> XXXXXXXXXXXXXXXXXXXXXXXXXXXXXXXXXXXXXXXXXXXXXXXXXXXXXXXXXXXXXXXXXXXXXXXXXXXXXXXXXXXXXXXXXXXXXXXXXXXXXXXXXXXXXXXXXXXXXXXXXXXXXXXXXXXXXXXXXXXXXXXXXXXXXXXXXXXXXXXXXXXXXXXXXXXXXXXXXXXXXXXXXXXXXXPSVPECFTIEKKSSYFIIEPQDLSTKVASICGVIVPKVHTIHDKVFYPLTFVPTHKTVSSLRQLGRKIQNSTPIMLIGKAGSGKTFLINELSKYMGCHDSIVKIHLGEQTDAKLLIGTYTSGDKPGTFEWRAGVLATAVKEGRWVLIEDIDKAPTDVLSILLSLLEKRELTIPSRGETVKAANGFQLISTVRINEDHQKDSSNKIYNLNMIGMRIWNVIELEEPSE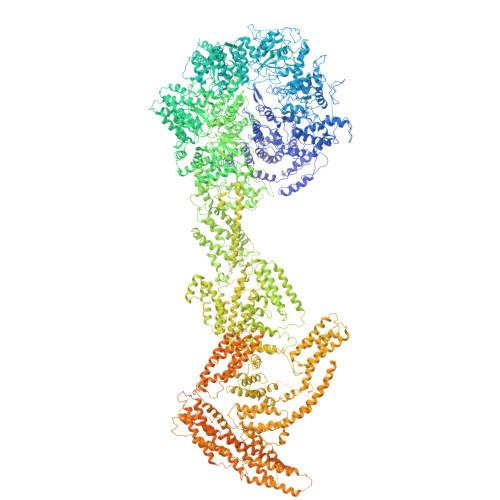EDLTHILAQKFPILTNLIPKLIDSYKNVKSIYMNTKFISLNKGAHTRVVSVRDLIKLCERLDILFKNNGINKPDQLIQSSVYDSIFSEAADCFAGAIGEFKALEPIIQAIGESLDIASSRISLFLTQHVPTLENLDDSIKIGRAVLLKEKLNIQKKSMNSTLFAFTNHSLRLMEQISVCIQMTEPVLLVGETGTGKTTVVQQLAKMLAKKLTVINVSQQTETGDLLGGYKPVNSKTVAVPIQENFETLFNATFSLKKNEKFHKMLHRCFNKNQWKNVVKLWNEAYKMAQSILKITNTENENENAKKKKRRLNTHEKKLLLDKWADFNDSVKKFEAQSSSIENSFVFNFVEGSLVKTIRAGEWLLLDEVNLATADTLESISDLLTEPDSRSILLSEKGDAEPIKAHPDFRIFACMNPATDVGKRDLPMGIRSRFTEIYVHSPERDITDLLSIIDKYIGKYSVSDEWVGNDIAELYLEAKKLSDNNTIVDGSNQKPHFSIRTLTRTLLYVTDIIHIYGLRRSLYDGFCMSFLTLLDQKSEAILKPVIEKFTLGRLKNVKSIMSQTPPSPGPDYVQFKHYWMKKGPNTIQEQAHYIITPFVEKNMMNLVRATSGKRFPVLIQGPTSSGKTSMIKYLADITGHKFVRINNHEHTDLQEYLGTYVTDDTGKLSFKEGVLVEALRKGYWIVLDELNLAPTDVLEALNRLLDDNRELFIPETQEVVHPHPDFLLFATQNPPGIYGGRKILSRAFRNRFLELHFDDIPQDELEIILRERCQIAPSYAKKIVEVYRQLSIERSASRLFEQKNSFATLRDLFRWALRDAVGYEQLAASGYMLLAERCRTPQEKVTVKKTLEKVMKVKLDMDQYYASLEDKSLEAIGSVTWTKGMRRLSVLVSSCLKNKEPVLLVGETGCGKTTICQLLAQFMGRELITLNAHQNTETGDILGAQRPVRNRSEIQYKLIKSLKTALNIANDQDVDLKELLQLYSKSDNKNIAEDVQLEIQKLRDSLNVLFEWSDGPLIQAMRTGNFFLLDEISLADDSVLERLNSVLEPERSLLLAEQGSSDSLVTASENFQFFATMNPGGDYGKKELSPALRNRFTEIWVPSMEDFNDVNMIVSSRLLEDLKDLANPIVKFSEWFGKKLGGGNATSGVISLRDILAWVEFINKVFPKIQNKSTALIQGASMVFIDALGTNNTAYLAENENDLKSLRTECIIQLLKLCGDDLELQQIETNEIIVTQDELQVGMFKIPRFPDAQSSSFNLTAPTTASNLVRVVRAMQVHKPILLEGSPGVGKTSLITALANITGNKLTRINLSEQTDLVDLFGADAPGERSGEFLWHDAPFLRAMKKGEWVLLDEMNLASQSVLEGLNACLDHRGEAYIPELDISFSCHPNFLVFAAQNPQYQGGGRKGLPKSFVNRFSVVFIDMLTSDDLLLIAKHLYPSIEPDIIAKMIKLMSTLEDQVCKRKLWGNSGSPWEFNLRDTLRWLKLLNQYSICEDVDVFDFVDIIVKQRFRTISDKNKAQLLIEDIFGKFSTKENFFKLTEDYVQINNEVALRNPHYRYPITQNLFPLECNVAVYESVLKAINNNWPLVLVGPSNSGKTETIRFLASILGPRVDVFSMNSDIDSMDILGGYEQVDLTRQISYITEELTNIVREIISMNMKLSPNATAIMEGLNLLKYLLNNIVTPEKFQDFRNRFNRFFSHLEGHPLLKTMSMNIEKMTEIITKEASVKFEWFDGMLVKAVEKGHWLILDNANLCSPSVLDRLNSLLEIDGSLLINECSQEDGQPRVLKPHPNFRLFLTMDPKYGELSRAMRNRGVEIYIDELHSRSTAFDRLTLGFELGENIDFVSIDDGIKKIKLNEPDMSIPLKHYVPSYLSRPCIFAQVHDILLLSDEEPIEESLAAVIPISHLGEVGKWANNVLNCTEYSEKKIAERLYVFITFLTDMGVLEKINNLYKPANLKFQKALGLHDKQLTEETVSLTLNEYVLPTVSKYSDKIKSPESLYLLSSLRLLLNSLNALKLINEKSTHGKIDELTYIELSAAAFNGRHLKNIPRIPIFCILYNILTVMSENLKTESLFCGSNQYQYYWDLLVIVIAALETAVTKDEARLRVYKELIDSWIASVKSKSDIEITPFLNINLEFTDVLQLSRGHSITLLWDIFRKNYPTTSNSWLAFEKLINLSEKFDKVRLLQFSESYNSIKDLMDVFRLLNDDVLNNKLSEFNLLLSKLEDGINELELISNKFLNKRKHYFADEFDNLIRYTFSVDTAELIKELAPASSLATQKLTKLITNKYNYPPIFDVLWTEKNAKLTSFTSTIFSSQFLEDVVRKSNNLKSFSGNQIKQSISDAELLLSSTIKCSPNLLKSQMEYYKNMLLSWLRKVIDIHVGGDCLKLTLKELCSLIEEKTASETRVTFAEYIFPALDLAESSKSLEELGEAWITFGTGLLLLFVPDSPYDPAIHDYVLYDLFLKTKTFSQNLMKSWRNVRKVISGDEEIFTEKLINTISDDDAPQSPRVYRTGMSIDSLFDEWMAFLSSTMSSRQIKELVSSYKCNSDQSDRRLEMLQQNSAHFLNRLESGYSKFADLNDILAGYIYSINFGFDLLKLQKSKDRASFQISPLWSMDPINISCAENVLSAYHELSRFFKKGDMEDTSIEKVLMYFLTLFKFHKRDTNLLEIFEAALYTLYSRWSVRRFRQEQEENEKSNMFKFNDNSDDYEADFRKLFPDYEDTALVTNEKDISSPENLDDIYFKLADTYISVFDKDHDANFSSELKSGAIITTILSEDLKNTRIEELKSGSLSAVINTLDAETQSFKNTEVFGNIDFYHDFSIPEFQKAGDIIETVLKSVLKLLKQWPEHATLKELYRVSQEFLNYPIKTPLARQLQKIEQIYTYLAEWEKYASSEVSLNNTVKLITDLIVSWRKLELRTWKGLFNSEDAKTRKSIGKWWFYLYESIVISNFVSEKKETAPNATLLVSSLNLFFSKSTLGEFNARLDLVKAFYKHIQLIGLRSSKIAGLLHNTIKFYYQFKPLIDERITNGKKSLEKEIDDIILLASWKDVNVDALKQSSRKSHNNLYKIVRKYRDLLNGDAKTIIEAGLLYXXXXXXXXXXXXXXXXXXXXXXXXXXXXXXXRNIDTVASNMDSYLEKISSQEFPNFADLASDFYAEAERLRKETPNVYTKENKKRLAYLKTQKSKLLGDALKELRRIGLKVNFREDIQKVQSSTTTILANIAPFNNEYLNSSDAFFFKILDLLPKLRSAASNPSDDIPVAAIERGMALAQSLMFSLITVRHPLSEFTNDYCKINGMMLDLEHFTCLKGDIVHSSLKANVDNVRLFEKWLPSLLDYAAQTLSVISKYSATSEQQKILLDAKSTLSSFFVHFNSSRIFDSSFIESYSRFELFINELLKKLENAKETGNAFVFDIIIEWIKANKGGPIKKEQKRGPSVEDVEQAFRRTFTSIILSFQKVIGDGIESISETDDNWLSASFKKVMVNVKLLRSSVVSKNIETALSLLKDFDFTTTESIYVKSVISFTLPVITRYYNAMTVVLERSRIYYTNTSRGMYILSTILHSLAKNGFCSPQPPSEEVDDKNLQEGTGLGDGEGAQNNNKDVEQDEDLTEDAQNENKEQQDKDERDDENEDDAVEMEGDMAGELEDLSNGEENDDEDTDSEEEELDEEIDDLNEDDPNAIDDKMWDDKASDNSKEKDTDQNLDGKNQEEDVQAAENDEQQRDNKEGGDEDPNAPEDGDEEIENDENAEEENDVGEQEDEVKDEEGEDLEANVPEIETLDLPEDMNLDSEHEESDEDVDMSDGMPDDLNKEEVGNEDEEVKQESGIESDNENDEPGPEEDAGETETALDEEEGAEEDVDMTNDEGKEDEENGPEEQAMSDEEELKQDAAMEENKEKGGEQNTEGLDGVEEKADTEDIDQEAAVQQDSGSKGAGADATDTQEQDDVGGSGTTQNTYEEDQEDVTKNNEESREEATAALKQLGDSMKEYHRRRQDIKEAQTNGEEDENLEKNNERPDEFEHVEGANTETDTQALGSATQDQLQTIDEDMAIDDDREEQEVDQKELVEDADDEKMDIDEEEMLSDIDAHDANNDVDSKKSGFIGKRKSEEDFENELSNEHFSADQEDDSEIQSLIENIEDNPPDASASLTPERSLEESRELWHKSEISTADLVSRLGEQLRLILEPTLATKLKGDYKTGKRLNMKRIIPYIASQFRKDKIWLRRTKPSKRQYQIMIALDDSKSMSESKCVKLAFDSLCLVSKTLTQLEAGGLSIVKFGENIKEVHSFDQQFSNESGARAFQWFGFQETKTDVKKLVAESTKIFERARAMVHNDQWQLEIVISDGICEDHETIQKLVRRARENKIMLVFVIIDGITSNESILDMSQVNYIPDQYGNPQLKITKYLDTFPFEFYVVVHDISELPEMLSLILRQYFTDLASS> MSPILGYWKIKGLVQPTRLLLEYLEEKYEEHLYERDEGDKWRNKKFELGLEFPNLPYYIDGDVKLTQSMAIIRYIADKHNMLGGCPKERAEISMLEGAVLDIRYGVSRIAYSKDFETLKVDFLSKLPEMLKMFEDRLCHKTYLNGDHVTHPDFMLYDALDVVLYMDPMCLDAFPKLVCFKKRIEAIPQIDKYLKSSKYIAWPLQGWQ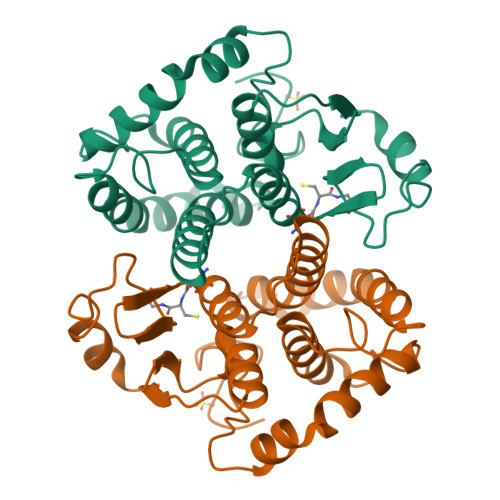ATFGGGDHPPK> NVSFPASVQLHTAVEMHHWCIPFSVDGQPAPSLRWLFNGSVLNETSFIFTEFLEPA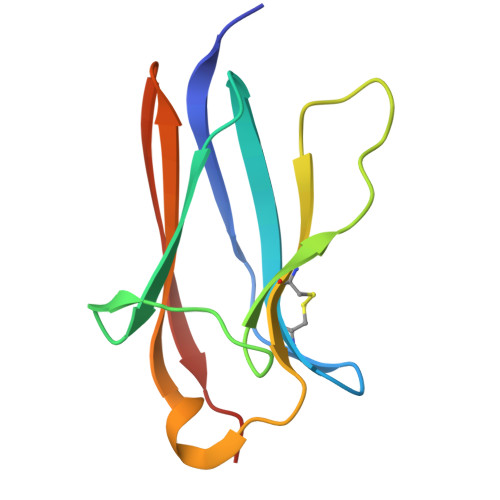ANETVRHGCLRLNQPTHVNNGNYTLLAANPFGQASASIMAAFMDNP>[4x]MAHHHHHHMRLCGFEAGLDKPLFLIAGPCVIESEELALETAGYLKEMCSQLNIPFIYKSSFDKANRSSISS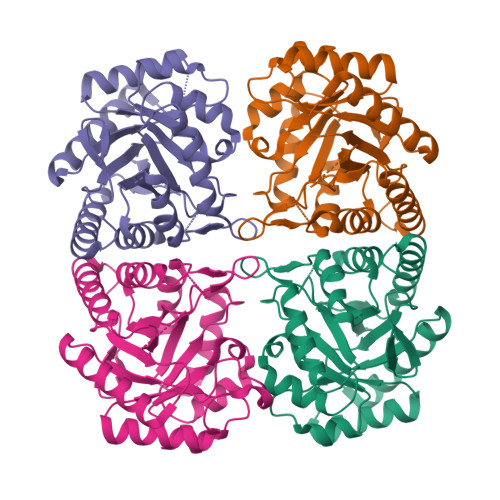YRGPGFEKGLSILEKVKSQIGVPVLTDVHEDTPLFEVSSVVDVLQTPAFLCRQTNFIQKVAAMNKPVNIKKGQFLAPWEMKHVIAKAKAQGNEQIMACERGVSFGYNNLVSDMRSLVIMRETGCPVVYDATHSVQLPGGNNGVSGGQREFIPALARAAVAVGISGLFMETHPDPDKALSDGPNSWPLDKMKQLLESLKAADEVYKKYSTDF(2S)-4-({[(2S,3S,4R,5R)-5-(6-amino-9H-purin-9-yl)-3,4-dihydroxytetrahydrofuran-2-yl]methyl}sulfanyl)-2-{[(2E)-3-(cis-4-hydroxycyclohexa-2,5-dien-1-yl)prop-2-enoyl]amino}butanoic acid | C23 H28 N6 O7 S | 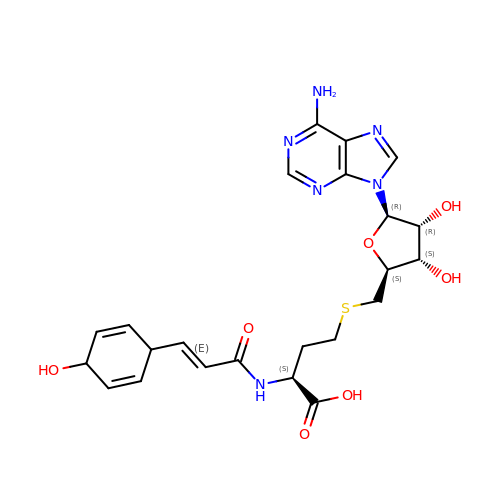MCKGCHUZDZFSOU-PDOWKVAKSA-N> MPSVYGARLTTFEDEEKESEYGYVRKVSGPVVIADGMNGAAMYELVRVGHDNL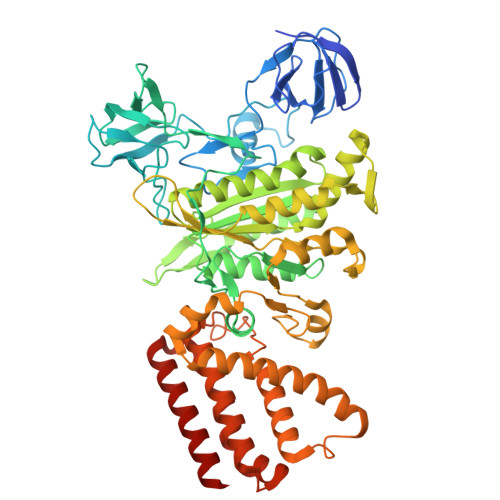IGEIIRLEGDSATIQVYEETAGLMVNDPVLRTHKPLSVELGPGILGNIFDGIQRPLKTIAIRSGDVYIPRGVSVPALDKDTLWEFQPKKIGEGDLLTGGDLYATVFENSLMQHHVALPPDAMGKVTYVAPAGQYSLKDTVLELEFQGVKKSFTMLQAWPVRTPRPVSSKLAADTPLLTGQRVLDALFPSVLGGTCAIPGAFGCGKTVISQALSKYSNSDTVVYVGCGERGNEMAEVLMDFPQLTMTLPDGREESVMKRTTLVANTSNMPVAAREASIYTGITIAEYFRDMGYNVSMMADSTSRWAEALREISGRLAEMPADSGYPAYLAARLASFYERAGKVKCLGGPERTGSVTIVGAVSPPGGDFSDPVTSATLSIVQVFWGLDKKLAQRKHFPSVNWLISYSKYSTALESFYEQFDPDFINIRTKAREVLQREDDLNEIVQLVGKDALAEGDKITLETAKLLREDYLAQNAFTPYDKFCPFYKSVWMMRNIIHFYNLANQAVEKGAGMDGQKITYTLIKHRLGDLFYRLVSQKFEDPAEGEPALVAKFKKLHEDLTAGFRALEDETR> SLSRLESENVKRLRQEKRLSLIVDLDQTIIHATVDPTVGEWMSDPGNVNYDVLRDVRSFNLQEGPSGYTSCYYIKFRPGLAQFLQKISELYELHIYTMGTKAYAKEVAKIIDPTGKLFQDRVLSRDDSGSLAQKSLRRLFPCDTSMVVVIDDRGDVWDWNPNLIKVVPYEFFVGIGDINSNFLSGNREALEEQNKERVTALELQKSERPLAKQQNALLEDEGKPTPSHTLLH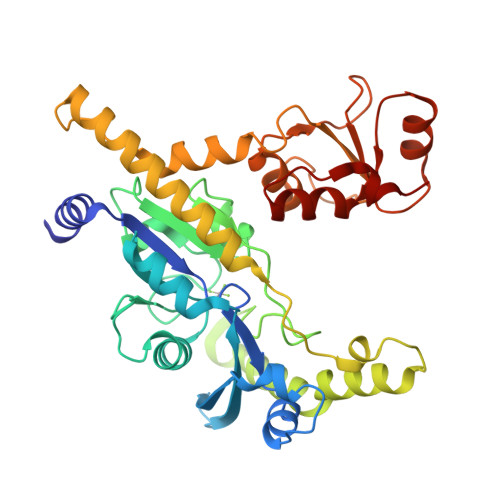NRDHELERLEKVLKDIHAVYYEEENDISSRSGNHKHANVGLIIPKMKQKVLKGCRLLFSGVIPLGVDVLSSDIAKWAMSFGAEVVLDFSVPPTHLIAAKIRTEKVKKAVSMGNIKVVKLNWLTESLSQWKRLPESDYLLY>MSDYKDDDDKGGGGSMAIAHLATEYVFSDFLLKEPTEPKFKGLRLELAVDKMVTCIAVGLPLLLISLAFAQEISIGTQISCFSPSSFSWRQAAFVDSYCWAAVQQKSSLQSESGNLPLWLHKFFPYILLLFAILLYLPALFWRFSAAPHLCSDLKFIMEELDKVYNRAIKAAKSARDLDLRDGPGPPGVTENVGQSLWEISESHFKYPIVEQYLKTKKNSSHLIMKYISCRLVTFVVILLACIYLSYYFSLSSLSDEFLCSIKSGVLKNDSTIPDRFQCKLIAVGIFQLLSLINLIVYALLIPVVVYTFFIPFRQKTDILKVYEILPTFDVLHFKSEGYNDLSLYNLFLEENISELKSYKCLKVLENIKSNGQGIDPMLLLTNLGMIKMDIIDGKIPTSLQTKGEDQGSQRVEFKDLDLSSEAAANNGEKNSRQRLLNPSCLEVLFQ[7x]

In this work, we present a case study using a streamlined version of the DirectMX protocol working directly from crude cell pellets to purify the ATP release channel pannexin1 (PANX1), and investigate its structural and ligand-binding properties. PANX1 is a potential therapeutic target and associated with various pathologies, including inflammation, pain, ischemia, and epilepsy. Several PANX1 structures have previously been solved and all of them approximately show similar overall structures albeit with differences in the intracellular domains15–22 and lipid-like densities at the membrane interface.

The cryo-EM structure of mouse PANX1 was solved (3.1 Å), representing the first published structure of a membrane protein extracted by Salipro nanoparticles directly from cells. Cryo-EM micrographs revealed that frozen-hydrated complexes were monodisperse with 2D class averages displaying secondary and tertiary structures, as well as heptameric organization of mPANX1. Extracellular and transmembrane regions of the Salipro-mPANX1 are well-resolved in the structure with clear side-chain density visible. In contrast, much of the intracellular regions were not well resolved in the cryo-EM map prohibiting complete atomic modelling. The dimensions of the Salipro-mPANX1 heptamer are 90 by 104 Å, which is slightly smaller than those of hPANX1, which are 96 by 109 Å. On the protomer level, the mouse and human PANX1 structures are highly similar, with a root-mean-square deviation (RMSD) of 1.556 across 256 aligned atom pairs. On the other hand, the N-terminus of Salipro-mPANX1 could not be resolved, similar to what has been reported for several other PANX1 structures. Furthermore, the structured intracellular region of Salipro-mPANX1 exhibits some minor but clear differences compared to the hPANX1 with several alpha-helices shifted; for example, helices encompassing residues 342–349 (Salipro-mPANX1) and 342–355 (hPANX1) reach a maximum displacement of ~ 5 Å. In addition, it was not possible to resolve any lipid-like density in the Salipro-mPANX1 structure. Since our structure contains endogenous lipids from mPANX1-expressing cells, this lack of lipid-like density could suggest that endogenous lipids have a certain flexibility surrounding mPANX1.>[4x]MNSKCHCVILNDGNFIPVLGFGTALPLECPKSKAKELTKIAIDAGFHHFDSASVYNTEDHVGEAIRSKIADGTVRREDIFYTSKVWCTSLHPELVRASLERSLQKLQFDYVDLYLIHYPMALKPGEENFPV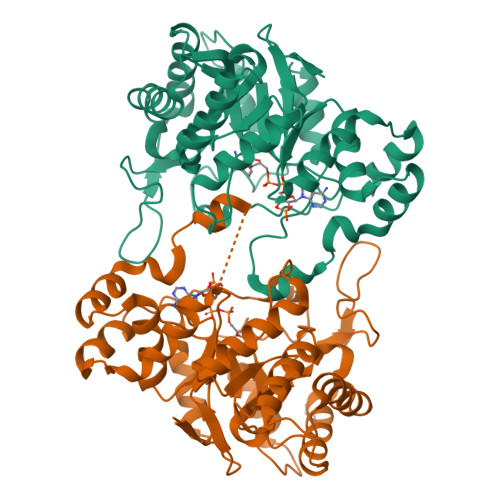DEHGKLIFDRVDLCATWEAMEKCKDAGLTKSIGVSNFNYRQLEMILNKPGLKYKPVCNQVECHPYLNQMKLLDFCKSKDIVLVAYGVLGTQRYGGWVDQNSPVLLDEPVLGSMAKKYNRTPALIALRYQLQRGIVVLNTSLKEERIKENMQVFEFQLSSEDMKVLDGLNRNMRYIPAAIFKGHPNWPFLDEY>[2x]AEKEKNAAEIRQQFAMTAGSPIIVNDKLERYAEVRTAFTHPTSFFKPNYKGEVKPWFLSAYDEKVRQIENGENGPKMKAKNVGEARAGRALEAAGWTLDINYGNIYPNRFFMLWSGETMTNTQLWAPVGLDRRPPDTTDPVELTNYVKFAARMAGADLVGVARLNRNW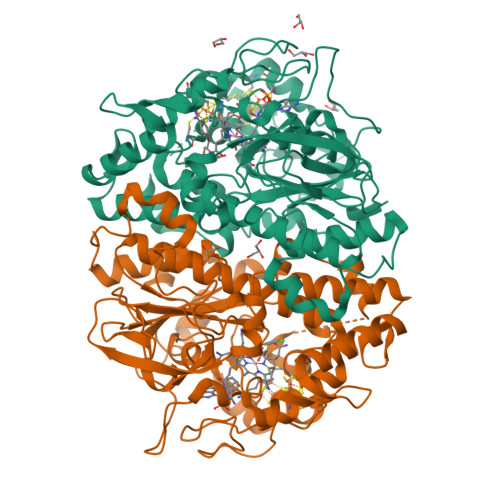VYSEAVTIPADVPYEQSLHKEIEKPIVFKDVPLPIETDDELIIPNTCENVIVAGIAMNREMMQTAPNSMACATTAFCYSRMCMFDMWLCQFIRYMGYYAIPSCNGVGQSVAFAVEAGLGQASRMGACITPEFGPNVRLTKVFTNMPLVPDKPIDFGVTEFCETCKKCARECPSKAITEGPRTFEGRSIHNQSGKLQWQNDYNKCLGYWPESGGYCGVCVAVCPFTKGNIWIHDGVEWLIDNTRFLDPLMLGMDDALGYGAKRNITEVWDGKINTYGLDADHFRDTVSFRKDRVKKS> MGSSHHHHHAMSEHRNEKGERISMINP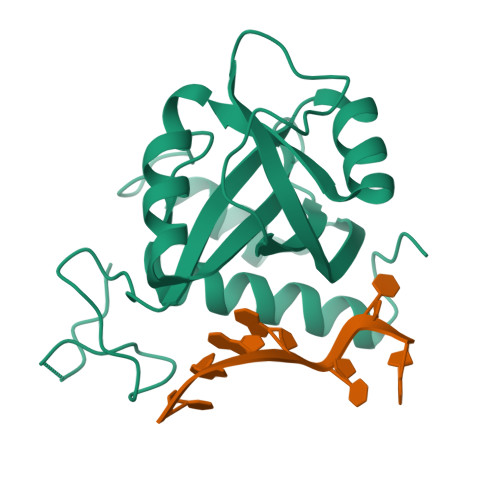RVVLDENGISHRSRYFIMLCDNETAIAHAKKTSIWAVKKDSSKRISDAYKKASVYFIFVAQQTYNALGYAQVVSDLNSTELPFWSDSSHAGGVRIKWIKTCNLFSAEISEIVSHMDHGSEARDGMEMMYDEGSRLCTLINYAIMKRIGRDR Viral occlusion bodies (OBs), also called polyhedra, are stable protein crystals that encapsulate newly assembled virions within virus-infected cells. The crystalline polyhedra is formed by repeating units of the ~27.5 kDa ToNV polyhedrin protein, which is predominantly helical, containing ten helices and a short two-stranded antiparallel beta sheet. The ToNV polyhedrin structure is almost completely helical, with a 3D fold not previously observed (to the best of our knowledge). The ToNV polyhedrin achieves the first requirement by forming a dense lattice, free from continuous channels, maintained in all directions by disulfide bonds, hydrophobic and electrostatic interactions, and domain swapping.

During initial analysis of individual crystals of recombinantly expressed polyhedrin, we noted the presence of a crystal population (approximately 10% of crystals which could be indexed) where the unit cell had increased by 3.5 Å in two directions, giving cell dimensions of a = b = 57.2 Å, c = 105.8 Å. These crystals diffracted weakly, yielding a dataset to approximately 2.8 Å. Analysis of the structure showed significant portions of the structure were disordered. Residues 143–191 could not be resolved in the electron density maps, with helix-α9 and the N-terminal region of helix-α10 disordered. The region between helix-α5 and helix-α7 was remodelled and helix-α6 was poorly resolved. At the N-terminus, only helix-α2 remained well resolved while the connecting loops and helix-α1 were not visible. The crystallographic disordering of these polyhedrin residues creates channels within the protein crystals. This increase in unit cell and the disordering of residues appears similar to that observed in a CPV4 polyhedra structure where similar changes occurred. Whether this crystal form represents an assembly or disassembly intermediate, or an artefact of purification is unclear.

> MGYLCNDYGYEPNVDYPNASHAGLYDRSKQPYVDTAIGPKTTIQFDHVFIKSDFKTWLAHNQDEAILLIRLYELGLLLQGRSDSFLEFYNNTTYITRTDSKQPFLNKYGKLVDTTSVTCLDIFLSVVLFALNQIDSLICDFKNTPWINLSKEHKKIYELVRGIFGICYGEKDYNRFEYCPFDANSTASALNVNATLNAKKTIELITCGLIRALIAYANLVTAFSADKTALLHEILLTKVCC> GPTSGSGPPRKVEVEPLNSTAVHVSWKLPVPNKQHGQIRGYQVTYVRLENGEPRGQPIIQDVMLAEAQETTISGLTPETTYSITVAAYTTKGDGARSKPKVVTTTGAVP

An understudied class of proteins in phosphotyrosine signaling, the receptor protein tyrosine phosphatases (RPTPs), are a family of single-pass transmembrane proteins whose architecture include an extracellular domain resembling those of cell adhesion molecules (CAMs) and intracellular single or tandem tyrosine phosphatase domains. In vertebrates, this diversity is typified by the leukocyte common antigen related (Lar) and its two homologs RPTPδ/PTPRD and RPTPσ/PTPRS, which form the type IIa family of RPTPs. The ectodomains of Lar-RPTPs resemble immunoglobulin (Ig)-superfamily CAMs and include three Ig-like domains followed by four to nine fibronectin type III (FN) repeats. Surprisingly, we uncovered a tripeptide, Lys-Gly-Asp (KGD), in the Dlar FN5 domain that is similar to the RGD motif in FN10 and is conserved in the Lar-RPTP homologs across species.

We sought to gain further insights into the position of the conserved KGD motif in mammalian homologues of Dlar. We thus determined the crystal structures of the FN5 domain of mouse LAR and the FN4-FN6 fragment of human RPTPδ. The LAR FN5 crystal structure was solved by molecular replacement using Dlar FN5 as the model and refined to a resolution of 1.7 Å, while the structure of the FN4-FN6 fragment was to a resolution of 1.77 Å. Overall, the LAR FN5 adopts a structure that is very similar to that of Dlar FN5. However, the KGD peptide remains poorly accessible and is thus unlikely to favor binding to integrin complexes. Thus, if Dlar and its mammalian homologues interact directly with integrins, they will use a mechanism that is distinct from the canonical RGD/integrin binding interaction. (C) A ribbon diagram of the FN5 domain of mouse Lar is shown in cyan. Residues in the mouse Lar KGD motif are shown in ball-and-stick representation.> GPMRTKIV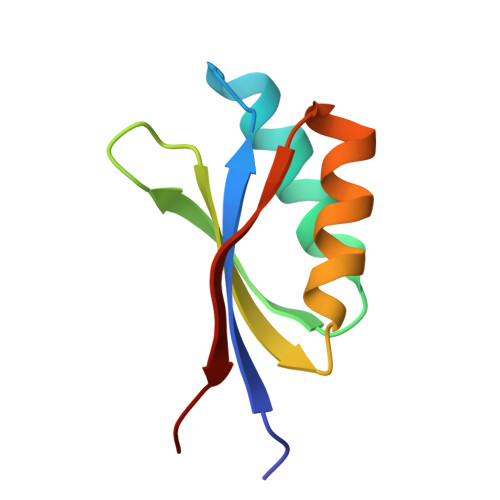VKVHMPCGKSRAKAMALAASVNGVDSVEITGDDKDRLQVVGRGIDPVRLVALLREKCGLAELLQVEEVKE> SNAASGSALIFDEEMSRYKLLWTDPECEIEVPERLTVSYEALRTHGLAQRCKAVPVRQATEQEILLAHSEEYLEAVKQTPGMNVEELMAFSKKYNAVYFHQNIYHCAKLAAGATLQLVDSVMKREVRNGMALVRPPGHHSQRSAANGFCVFNNVAFA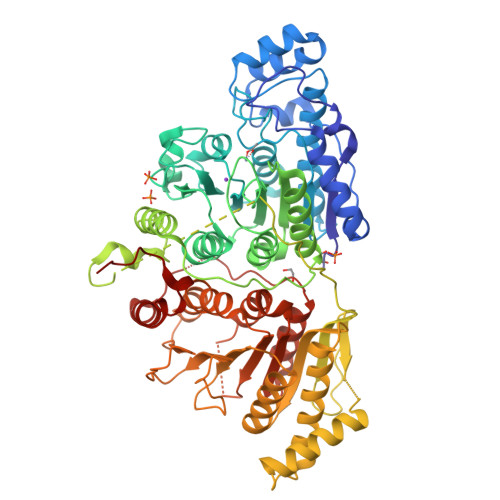ALYAKKNYNLNRILIVDWDVHHGQGIQYCFEEDPSVLYFSWHRYEHQSFWPNLPESDYSSVGKGKGSGFNINLPWNKVGMTNSDYLAAFFHVLLPVAYEFDPELVIVSAGFDSAIGDPEGEMCALPEIFAHLTHLLMPLAAGKMCVVLEGGYNLTSLGQSVCQTVHSLLGDPTPRISGLGTACDSALESIQNVRNVQSSYWSSFKHLAQSETNPKRPRLDATNGGPKESSEPASESNPKKTAQDDVWPEPLKRMPASVRTVVVPPPGVELTLPKNCQHSGDISESTAKEVQRIRDKHFHDLTDQNILRSLGNIISVLDRMMRSDEVCNGCVVVSDLSVSVQCALQHALTEPAERVLVVYVGDGELPVKTNDGKVFLVQICTKETEDKCVNRLTLCLREGESLTAGFMQALLGLILPVAYEFNPALVLGIVEETAAKTRLMRVWGHMTCLIQGLARGRMLTLLQGYDKDLLELTVSALSGASISPLGPLRAPKPEDVEMMEKQRQRLQERWGLLRCTVSESW>[2x]MRTELLSKLYDDFGIDQLPHTQHGVTSDRLGKLYEKYILDIFKDIESLKKYNTNAFPQEKDISSKLLKALNLDLDNIIDVSSSDTDLGRTIAGGSPKTDATIRFTFHNQSSRLVPLNIKHSSKKKVSIAEYDVETICTGVGISDGELKELIRKHQNDQSAKLFTPVQKQRLTELLEP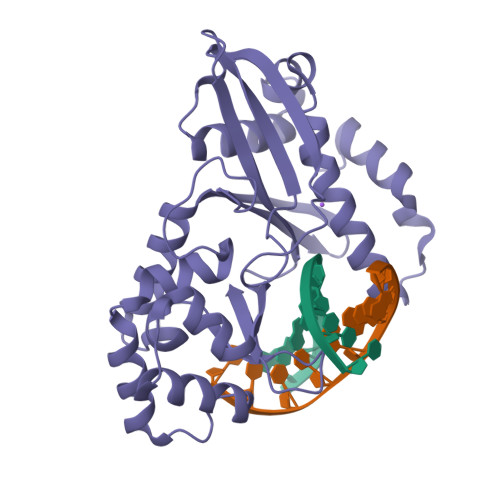YRERFIRWCVTLRAEKSEGNILHPDLLIRFQVIDREYVDVTIKNIDDYVSDRIAEGSKARKPGFGTGLNWTYASGSKAKKMQFKG>[4x]FQKIYSPTQLANAMKLVRQQNGWTQSELAKKIGIKQATISNFENNPDNTTLTTFFKILQSLELSMTLCDAK;>PKLVTWMNNQRVGELTKLANGAHTFKYAPEWLASRYARPLSLSLPLQRGNITSDAVFNFFDNLLPDSPIVRDRIVKRYHAKSRQPFDLLSEIGRDSVGAVTLIPEDETVTHPIMAWEKLTEARLEEVLTAYKADIPLGMIREENDFRISVAGAQEKTALLRIGNDWCIPKGITPTTHIIKLPIGEIRQPNATLDLSQSVDNEYYCLLLAKELGLNVPDAEIIKAGNVRALAVERFDRRWNAERTVLLRLPQEDMCQTFGLPSSVKYESDGGPGIARIMAFLMGSSEALKDRYDFMKFQVFQWLIGATQGHAKNFSVFIQAGGSYRLTPFYDIISAFPVLGGTGIHISDLK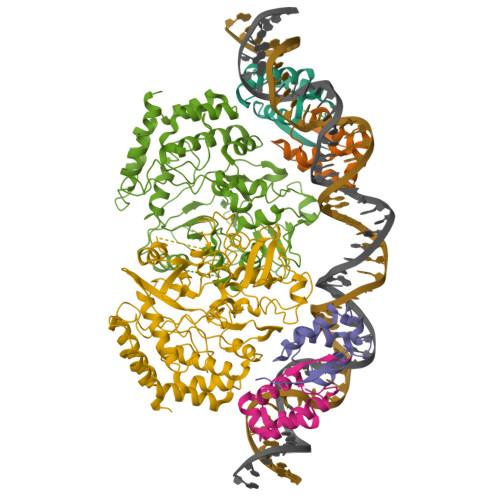LAMGLNASKGKKTAIDKIYPRHFLATAKVLRFPEVQMHEILSDFARMIPAALDNVKTSLPTDFPENVVTAVESNVLRLHGRLSREY[2x]> SDVRPPHILVKTLDYIVDNLLTTLPESEGFLWDRMRSIRQDF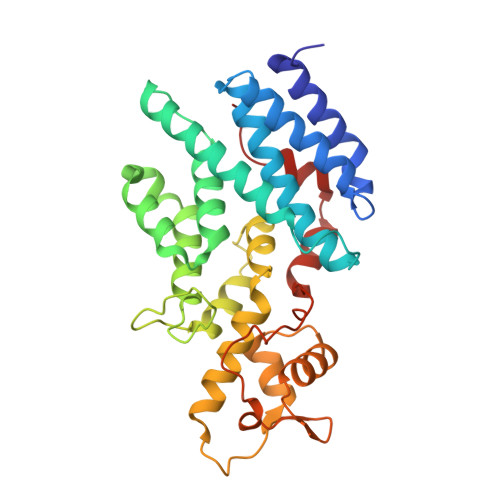TYQNYSGPEAVDCNERIVRIHLLILHIMVKSNVEFSLQQELEQLHKSLITLSEIYDDVRSSGGTCPNEAEFRAYALLSKIRDPQYDENIQRLPKHIFQDKLVQMALCFRRVISNSAYTERGFVKTENCLNFYARFFQLMQSPSLPLLMGFFLQMHLTDIRFYALRALSHTLNKKHKPIPFIYLENMLLFNNRQEIIEFCNYYSIEIINGDAADLKTLQHYSHKLSETQPLKKTYLTCLERRLQKTTYKGLINGGEDN> MLTEGITIQSYDGHTFGALVGSPVKAPAPVIVIAHEILGVNAFMRETVSWLVDQGYAAVCPDLYARQAPGTALDPQDEAQREQAYKLWQAFDMEAGVGDLEAAIRYARHLPYSNGKVGLVGYSLGGALAFLVAAKGYVDRAVGYCGVGLEKQLNKVPEVKHPALFHMGGQDHFVPAPSRQLITEGFGANPLLQVHWYEGAGHSFA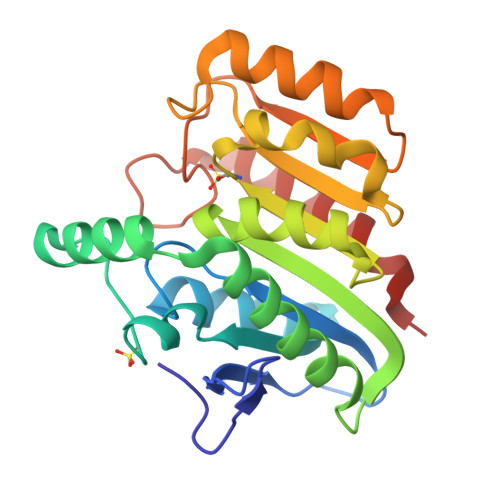RTGSSGYVASAAALANERTLDFLAPLQSKKP>MSHYKSNVRDQVFNLFEVFGVDKVLGADKFSDLDADTAREMLTEIARLAEGPIAESFVEGDRNPPVFDPETHTVTLPEGFKKSMRALFDGGWDKVGLAEHLGGIPMPRALQWALIEHILGANPAAYMYAMGPGMSEIFYNNGTDEQKKWATIAAERGWGATMVLTEPDAGSDVGAGRTKAVQQPDGTWHIEGVKRFITSADSDDLFENIMHLVLARPEGAGPGTKGLSLFFVPKFHFDHETGEIGERNGVFVTNVEHKMGLKVSATCELSLGQHGIPAVGWLVGEVHNGIAQMFDVIEQARMMVGTKAIATLSTGYLNALEYAKERVQGADMTQMTDK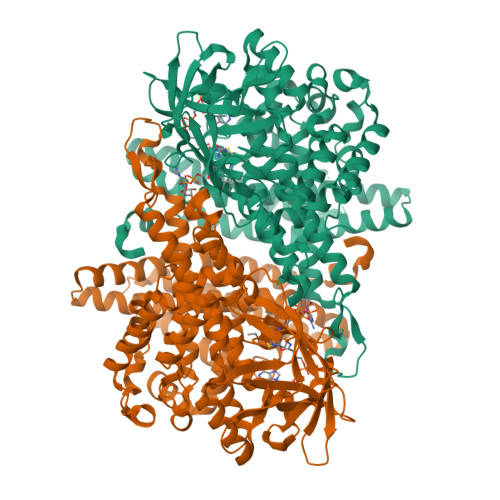TAPRVTITHHPDVRRSLMTQKAYAEGLRAIYLYTATFQDAEVAQAVHGVDGDLAARVNDLLLPIVKGFGSETAYAKLTESLQTLGGSGFLQDYPIEQYIRDSKIDSLYAGTTAIQAQDFFFRKIIRDKGQALAYVAGEIEQFIKNENGNGRLKTERELLATALADVQGMAASLTGYLMAAQEDAASIYKVGLGSVRFLMAVGDLLSGWLLARQAAVAIEKLDAGATGADKSFYEGKIAAASFFAKNMLPLLTSTRQIIENLDNDVMELDEAAF[2x]>MHHHHHHLTKVFGSRNDRTLRRMRKVVNIINAMEPEMEKLSDEELKGKTAEFRARLEKGEVLENLIPEAFAVVREASKRVFGMRHFDVQLLGGMVLNERCIAEMRTGEGKTLTATLPAYLNALTGKGVHVVTVNDYLAQRDAENNRPLFEFLGLTVGINLPGMPAPAKREAYAADITYGTNNEYGFDYLRDNMAFSPEERVQRKLHYALV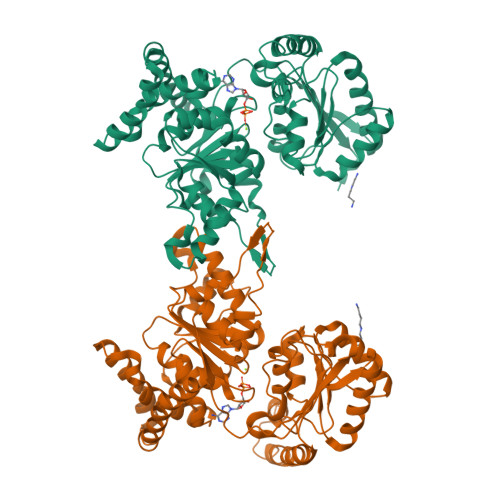DEVDSILIDEARTPLIISGANQTLASITFQNYFRLYEKLAGMTGTADTEAFEFSSIYKLDTVVVPTNRPMIRKDLPDLVYMTEAEKIQAIIEDIKERTAKGQPVLVGTISIEKSELVSNELTKAGIKHNVLNAKFHANEAAIVAQAGYPAAVTIATNMAGRGTDIVLGGSWQAEVAALENPTAEQIEKIKADWQVRHDAVLEAGGLHIIGTERHESRRIDNQLRGRSGRQGDAGSSRFYLSMEDALMRIFASDRVSGMMRK[2x]> MAFKFKTFAAVGALIGSLALVGCGQDEKDPNHIKVGVIVGAEQQVAEVAQKVAKDKYGLDVELVTFNDYVLPNEALSKGDIDANAFQHKPYLDQQLKDRGYKLVAVGNTFVYPIAGYSKKIKSLDELQDGSQVAVPNDPTNLGRSLLLLQKVGLIKLKDGVGLLPTVLDVVENPKNLKIVELEAPQLPRSLDDAQIALAV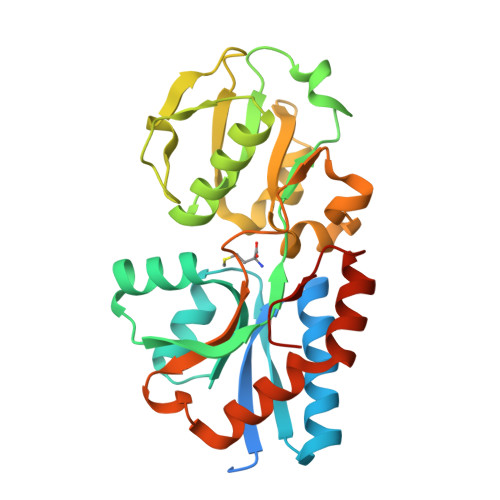INTTYASQIGLTPAKDGIFVEDKESPYVNLIVTREDNKDAENVKKFVQAYQSDEVYEAANKVFNGGAVKGWLEHHHHHH>[2x]QQAGTETEEYHLPLTWERDGSSVSASVVIDSNWRWTHSTEDTTNCYDGNEWDSTLCPDADTCTENCAIDGVDQGTWGDTYGITASGSKLTLSFVTEGEYSTDIGSRVFLMADDDNYEIFNLLDKEFSFDVDASNLPCGLNGALY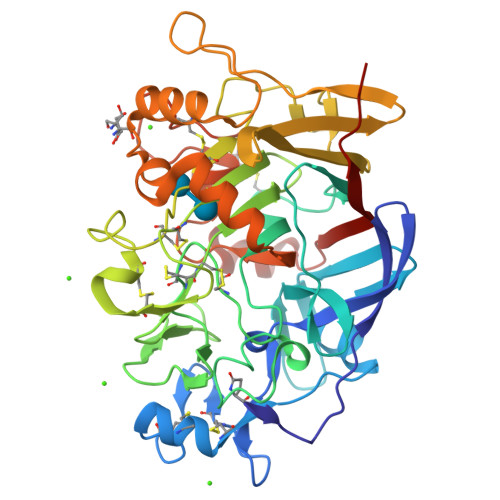FVSMDEDGGTSKYSTNTAGAKYGTGYCDAQCPHDMKFIAGKANSDGWTPSDNDQNAGTGEMGACCHEMDIWEANSQAQSYTAHVCSVDGYTPCTGTDCGDNGDDRYKGVCDKDGCDYAAYRLGQHDFYGEGGTVDSGSTLTVITQFITGGGGLNEIRRIYQQGGQTIQNAAVNFPGDVDPYDSITEDFCVDIKRYFGDTNDFDAKGGMSGMSNALKKGMVLVMSLWDDHYANMLWLDATYPVDSTEPGALRGPCSTDSGDPADVEANFPGSTVTFSNIKIGPIQSYD>AVDFSAHPWKAPGPNDSRGPCPGLNTLANHGFLPRNGRNISVPMIVKAGFEGYNVQSDILILAGKIGMLTSREADTISLEDLKLHGTIEHDASLSREDVAIGDNLHFNEAIFTTLANSNPGADVYNISSAAQVQHDRLADSLARNPNVTNTDLTATIRSSESAFFLTVMSAGDPLRGEAPKKFVNVFFREERMPIKEGWKRSTTPITIPLLGPIIERITELSDWKPTGDNCGAIVLSPE[4x]

Unspecific peroxygenases (UPOs) are enzymes catalyzing the oxyfunctionalization of both aromatic and aliphatic molecules, including specific products that are difficult to be obtained only by chemical means. Therefore, they are of high biotechnological interest for the regio- and/or stereoselective synthesis of biobased compounds and other fine chemicals and pharmaceuticals. These enzymes form a group of fungal heme-thiolate peroxidases (HTPs). Hence, they share a proximal cysteine residue acting as the fifth ligand of the heme iron with the phylogenetically distant cytochrome P450 monooxygenases (P450s), present in all living organisms. In the present study, two UPOs from the basidiomycete Marasmius rotula (rMroUPO) and the ascomycete Collariella virescens (rCviUPO) were crystallized after sequence optimization and Escherichia coli expression as active soluble enzymes.

The asymmetric unit of the rMroUPO crystal structure includes four polypeptide chains that associate to form a tetramer composed of two homo-dimers in a head-to-tail arrangement, each of them stabilized by an intermolecular disulfide bridge (between the Cys227 residue of both molecules). Each of the rMroUPO monomers is compact and spherical in shape and consists of residues from Ser1 to Glu235, which displayed clearly defined electron density (only lacking the C-terminal Leu236), together with one heme molecule and one Mg2+ ion. The overall fold is mainly helical with eleven α-helices and two short β-strands (V120-N122 and E174-P176). Moreover, a clear electron density could be detected at the active site that could be unequivocally assigned to an acetate ion from the crystallization medium. The heme cofactor sits in an internal pocket with its iron ion coordinated by the sulfur atom of rMroUPO Cys17 at a distance of 2.4 Å in the lower (also known as proximal because of the cysteine ligand) side of the heme cofactor. One of the acetate oxygens is near the sixth coordination position of the heme iron. The Mg2+ ion appears coordinated (at 2.07–2.19 Å distances) by the Ser89 hydroxyl, the His86 (backbone) carbonyl, two water molecules (wat1 and wat2), and the carboxylates of Glu85 and heme ring-D propionate (neighbor Asp87 is not involved in Mg2+ coordination). In rMroUPO, the dimer interface buries 825 Å2 of each monomer and is formed from the interactions between residues of the C-terminal loop and residues from the helix α4. From the C-terminal region, an intermolecular disulfide bond between the sulfhydryl side chains of Cys227 and the hydrophobic interactions established by Ile230 and Leu232 contribute to the clustering of the dimer. In addition, residues Ile62-Glu69 from the helix α4 increase the dimer stability by polar interactions of Lys61 with Ser67 and Glu69, and by a patch of hydrophobic residues at the interface (Ile62, Leu65).> MGSSHHHHHHSQDPNSNQAQELNHELELEQLETKITVSSVSLTGSTLNVVLENNGSTNLYDFQGFSVIV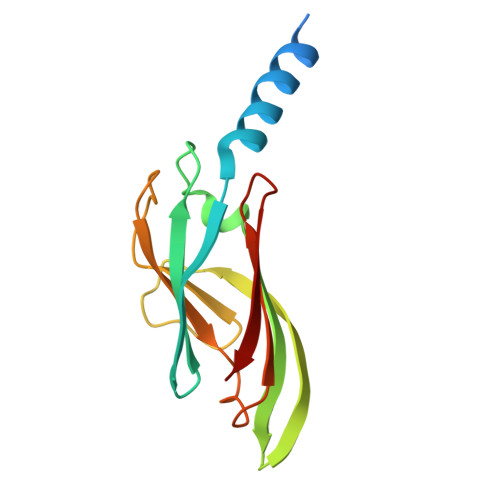QYYANISNISTFNLSLYNYTKNSNPSPYYWTINTPLLAPGSQATLTIILPYPPYPNTQATVVIVTNYGPSVIWRGSL>[2x]SSYRQARWWAQEITELAQGPGRDFLQLHRHDSYAPPRPGTLARWFVNGAGYFAAVADAILRAQEEIFITDWWLSPEVYLKRPAHSDDWRLDIMLKRKAEEGVRVSILLFKEVELALGINSGYSKRALMLLHPNIKVMRHPDQVTLWAHHEKLLVVDQVVAFLGGLDLAYGRWDDLHYRLTDLGDSSESAASQPPTPRPDSPATPDLSHNQFFWLGKDYSNLITKDWVQLDRPFEDFIDRETTPRMPWRDVGVVVHGLPARDLARHFIQRWNFTKTTKAKYKTPTYPYLLPKSTSTANQLPFTLPGGQCTTVQVLRSVDRWSAGTLENSILNAYLHTIRESQHFLY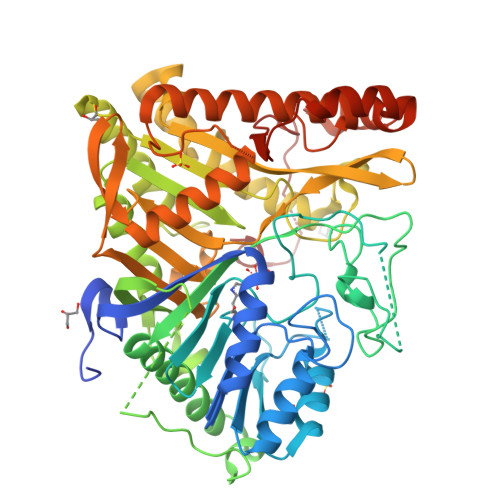IENQFFISCSDGRTVLNKVGDEIVDRILKAHKQGWCYRVYVLLPLLPGFEGDISTGGGNSIQAILHFTYRTLCRGEYSILHRLKAAMGTAWRDYISICGLRTHGELGGHPVSELIYIHSKVLIADDRTVIIGSANINDRSLLGKRDSELAVLIEDTETEPSLMNGAEYQAGRFALSLRKHCFGVILGANTRPDLDLRDPICDDFFQLWQDMAESNANIYEQIFRCLPSNATRSLRTLREYVAVEPLATVSPPLARSELTQVQGHLVHFPLKFLEDESLLPPLGSKEGMIPLEVWT> SNAMADKIKVGLLGYGYASKTFHAPLIMGTPGLELAGVSSSDASKVHADWPAIPVVSDPQMLFNDPSIDLIVIPTPNDTHFPLAQSALAAGKHVVVDKPFTVTLSQANALKEHADDAGLLLSVFHNRRWDSDFLTLKTLLAEGSLGNVVYFESHFDRYRPEIRQRWREQAGAGGGIWYDLGPHLLDQALQLFGLPETLNVDLGMLRPGSQSVDYFHAVLSYPGQRVVLHSTVLAAAETARYIVHGTQGSYIKFGVDPQEDRLKAGERLPQADWGYDMRDGIVTLSHDNVLTEKPLLTLPGNYPAYYA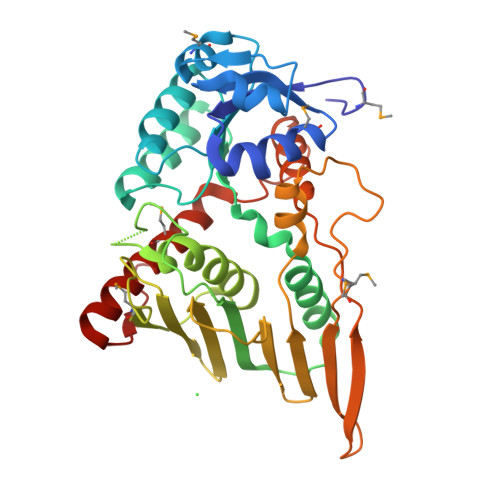GIRDAIWGTAPNPVPATEAIKVMELIELGIASDQQKKALPIIAKN>[6x]EGSPRLVLRALENMVRAAHT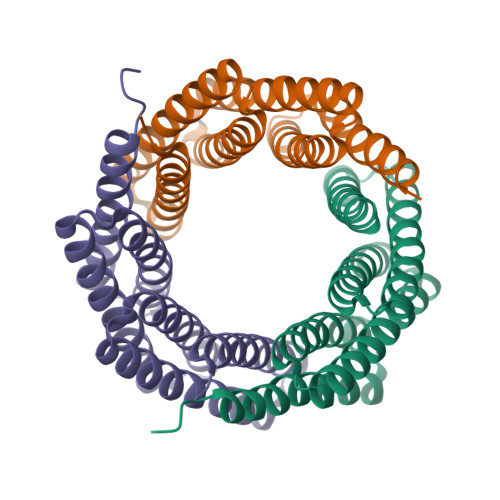LAEIARDNGNEEWLERAARLAEEVARRAEELAREARKEGNLELALKALQILVNAAYVLAEIARDRGNEELLEKAARLAEEAARQAEEIARQARKEGNFELALEALEILNEAARVLARIAHHRGNQELLEKAWRLTHRSAKWSREIAEQARKEGE>[8x]AAIVPTRELENVFLGRCKDYEITRYLDILPRVRSDCSALWKDFFKAFSFKNPCDLDLGSYKDFFTSAQQQLPKNKVMFWSGVYDEAHDYANTGRKYITLEDTLPGYMLNSLVWCGQRANPGFNEKVCPDFKTCP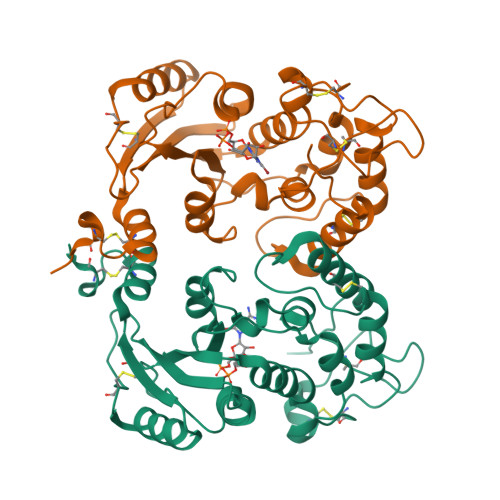VQARESFWGMASSSYAHSAEGEVTYMVDGSNPKVPAYRPDSFFGKYELPNLTNKVTRVKVIVLHRLGEKIIEKCGAGSLLDLEKLVKAKHFAFDCVENPRAVLFLLCSDNPNARECRLAKRFYRIA>MSELEKAVVALIDVFHQYSGREGDKHKLKKSELKELINNELSHFLEEIKEQEVVDKVMETLDSNGDGECDFQEFMAFVAMITTACHEFFEHE[2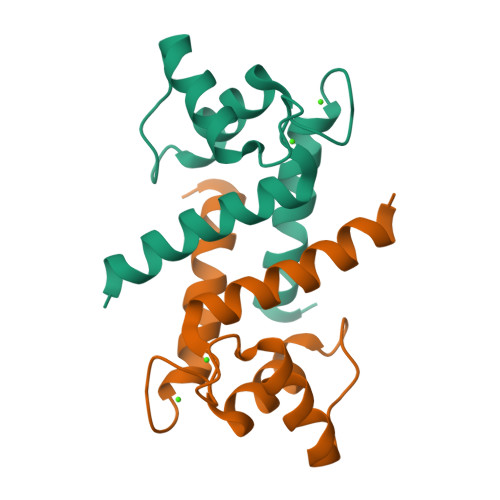x]The AAA+ (ATPases Associated with various cellular Activities) family member Rea1 (or Midasin) consists of nearly 5000 amino acids and generates force to mechanically remove assembly factors. Rea1 consists of an N-terminal α-helical domain (NTD), a ring of six AAA+ domains, and the C-terminal tail. The Rea1 tail is subdivided into an α-helical linker region, a D/E-rich region, and a MIDAS (Metal-Ion-Dependent Adhesion Site) domain which is responsible for the interaction with the Ytm1 and Rsa4 substrates. Rea1 pulls out the Ytm1 complex to promote the transfer of pre-60S particles from the nucleolus to the nucleoplasm.

In order to gain insight into the molecular basis for MIDAS domain docking, we decided to determine the cryoEM structure of the Rea1_ΔAAA2L-H2α AMPPNP state. The overall resolution of the reconstruction was 7.8 Å. The reconstruction revealed a density consistent with a MIDAS domain in-between the AAA3 and AAA4 modules, above AAA2S and AAA3S, respectively. As in the case of the Rea1_ΔAAA2L-H2α APO state, docking of this structure into the Rsa4 containing pre-60S structure would place the MIDAS domain in close contact with its Rsa4 substrate. Since the auto-inhibitory AAA2L-H2α insert has been deleted, the presence of AMPPNP is able to induce movements between the AAA+ modules of the AAA+ ring. The NTD, AAA1, AAA6 and the linker can be superimposed as a single rigid body, whereas the AAA2-AAA5 part has moved. The most drastic difference is apparent for the AAA4 module. Since the AAA2L-H2α insert is no longer pushing against AAA4L, the AAA4 module is free to move towards the central pore of the ring. We interpret these densities as two α-helices of the previously disordered AAA4L-H2α insert. The consequence of the combined movements of the AAA4 and AAA3 modules is that their small domains, AAA3S and AAA2S, adopt the right orientation with respect to each other to from the MIDAS domain binding site.

> XXXXXXXXXXXXXXXXXXXXXXXXXXXXXXXXXXXXXXXXXXXXXXXXXXXXXXXXXXXXXXXXXXXXXXXXXXXXXXXXXXXXXXXXXXXXXXXXXXXXXXXXXXXXXXXXXXXXXXXXXXXXXXXXXXXXXXXXXXXXXXXXXXXXXXXXXXXXXXXXXXXXXXXXXXXXXXXXXXXXXXXXXXXXXXPSVPECFTIEKKSSYFIIEPQDLSTKVASICGVIVPKVHTIHDKVFYPLTFVPTHKTVSSLRQLGRKIQNSTPIMLIGKAGSGKTFLINELSKYMGCHDSIVKIHLGEQTDAKLLIGTYTSGDKPGTFEWRAGVLATAVKEGRWVLIEDIDKAPTDVLSILLSLLEKRELTIPSRGETVKAANGFQLISTVRINEDHQKDSSNKIYNLNMIGMRIWNVIELEEPSEEDLTHILAQKFPILTNLIPKLIDSYKNVKSIYMNTKFISLNKGAHTRVVSVRDLIKLCERLDILFKNNGINKPDQLIQSSVYDSIFSEAADCFAGAIGEFKALEPIIQAIGESLDIASSRISLFLTQHVPTLENLDDSIKIGRAVLLKEKLNIQKKSMNSTLFAFTNHSLRLMEQISVCIQMTEPVLLVGETGTGKTTVVQQLAKMLAKKLTVINVSQQTETGDLLGGYKPVNSKTVAVPIQENFETLFNATFSLKKNEKFHKMLHRCFNKNQWKNVVKLWNEAYKMAQSILKITNTENENENAKKKKRRLNTHEKKLLLDKWADFNDSVKKFEAQSSSIENSFVFNFVEGSLVKTIRAGEWLLLDEVNLATADTLESISDLLTEPDSRSILLSEKGDAEPIKAHPDFRIFACMNPATDVGKRDLPMGIRSRFTEIYVHSPERDITDLLSIIDKYIGKYSVSDEWVGNDIAELYLEAKKLSDNNTIVDGSNQKPHFSIRTLTRTLLYVTDIIHIYGLRRSLYDGFCMSFLTLLDQKSEAILKPVIEKFTLGRLKNVKSIMSQTPPSPGPDYVQFKHYWMKKGPNTIQEQAHYIITPFVEKNMMNLVRATSGKRFPVLIQGPTSSGKTSMIKYLADITGHKFVRINNHEHTDLQEYLGTYVTDDTGKLSFKEGVLVEALRKGYWIVLDELNLAPTDVLEALNRLLDDNRELFIPETQEVVHPHPDFLLFATQNPPGIYGGRKILSRAFRNRFLELHFDDIPQDELEIILRERCQIAPSYAKKIVEVYRQLSIERSASRLFEQKNSFATLRDLFRWALRDAVGYEQLAASGYMLLAERCRTPQEKVTVKKTLEKVMKVKLDMDQYYASLEDKSLEAIGSVTWTKGMRRLSVLVSSCLKNKEPVLLVGETGCGKTTICQLLAQFMGRELITLNAHQNTETGDILGAQRPVRNRSEIQYKLIKSLKTALNIANDQDVDLKELLQLYSKSDNKNIAEDVQLEIQKLRDSLNVLFEWSDGPLIQAMRTGNFFLLDEISLADDSVLERLNSVLEPERSLLLAEQGSSDSLVTASENFQFFATMNPGGDYGKKELSPALRNRFTEIWVPSMEDFNDVNMIVSSRLLEDLKDLANPIVKFSEWFGKKLGGGNATSGVISLRDILAWVEFINKVFPKIQNKSTALIQGASMVFIDALGTNNTAYLAENENDLKSLRTECIIQLLKLCGDDLELQQIETNEIIVTQDELQVGMFKIPRFPDAQSSSFNLTAPTTASNLVRVVRAMQVHKPILLEGSPGVGKTSLITALANITGNKLTRINLSEQTDLVDLFGADAPGERSGEFLWHDAPFLRAMKKGEWVLLDEMNLASQSVLEGLNACLDHRGEAYIPELDISFSCHPNFLVFAAQNPQYQGGGRKGLPKSFVNRFSVVFIDMLTSDDLLLIAKHLYPSIEPDIIAKMIKLMSTLEDQVCKRKLWGNSGSPWEFNLRDTLRWLKLLNQYSICEDVDVFDFVDIIVKQRFRTISDKNKAQLLIEDIFGKFSTKENFFKLTEDYVQINNEVALRNPHYRYPITQNLFPLECNVAVYESVLKAINNNWPLVLVGPSNSGKTETIRFLASILGPRVDVFSMNSDIDSMDILGGYEQVDLTRQISYITEELTNIVREIISMNMKLSPNATAIMEGLNLLKYLLNNIVTPEKFQDFRNRFNRFFSHLEGHPLLKTMSMNIEKMTEIITKEASVKFEWFDGMLVKAVEKGHWLILDNANLCSPSVLDRLNSLLEIDGSLLINECSQEDGQPRVLKPHPNFRLFLTMDPKYGELSRAMRNRGVEIYIDELHSRSTAFDRLTLGFELGENIDFVSIDDGIKKIKLNEPDMSIPLKHYVPSYLSRPCIFAQVHDILLLSDEEPIEESLAAVIPISHLGEVGKWANNVLNCTEYSEKKIAERLYVFITFLTDMGVLEKINNLYKPANLKFQKALGLHDKQLTEETVSLTLNEYVLPTVSKYSDKIKSPESLYLLSSLRLLLNSLNALKLINEKSTHGKIDELTYIELSAAAFNGRHLKNIPRIPIFCILYNILTVMSENLKTESLFCGSNQYQYYWDLLVIVIAALETAVTKDEARLRVYKELIDSWIASVKSKSDIEITPFLNINLEFTDVLQLSRGHSITLLWDIFRKNYPTTSNSWLAFEKLINLSEKFDKVRLLQFSESYNSIKDLMDVFRLLNDDVLNNKLSEFNLLLSKLEDGINELELISNKFLNKRKHYFADEFDNLIRYTFSVDTAELIKELAPASSLATQKLTKLITNKYNYPPIFDVLWTEKNAKLTSFTSTIFSSQFLEDVVRKSNNLKSFSGNQIKQSISDAELLLSSTIKCSPNLLKSQMEYYKNMLLSWLRKVIDIHVGGDCLKLTLKELCSLIEEKTASETRVTFAEYIFPALDLAESSKSLEELGEAWITFGTGLLLLFVPDSPYDPAIHDYVLYDLFLKTKTFSQNLMKSWRNVRKVISGDEEIFTEKLINTISDDDAPQSPRVYRTGMSIDSLFDEWMAFLSSTMSSRQIKELVSSYKCNSDQSDRRLEMLQQNSAHFLNRLESGYSKFADLNDILAGYIYSINFGFDLLKLQKSKDRASFQISPLWSMDPINISCAENVLSAYHELSRFFKKGDMEDTSIEKVLMYFLTLFKFHKRDTNLLEIFEAALYTLYSRWSVRRFRQEQEENEKSNMFKFNDNSDDYEADFRKLFPDYEDTALVTNEKDISSPENLDDIYFKLADTYISVFDKDHDANFSSELKSGAIITTILSEDLKNTRIEELKSGSLSAVINTLDAETQSFKNTEVFGNIDFYHDFSIPEFQKAGDIIETVLKSVLKLLKQWPEHATLKELYRVSQEFLNYPIKTPLARQLQKIEQIYTYLAEWEKYASSEVSLNNTVKLITDLIVSWRKLELRTWKGLFNSEDAKTRKSIGKWWFYLYESIVISNFVSEKKETAPNATLLVSSLNLFFSKSTLGEFNARLDLVKAFYKHIQLIGLRSSKIAGLLHNTIKFYYQFKPLIDERITNGKKSLEKEIDDIILLASWKDVNVDALKQSSRKSHNNLYKIVRKYRDLLNGDAKTIIEAGLLYXXXXXXXXXXXXXXXXXXXXXXXXXXXXXXXRNIDTVASNMDSYLEKISSQEFPNFADLASDFYAEAERLRKETPNVYTKENKKRLAYLKTQKSKLLGDALKELRRIGLKVNFREDIQKVQSSTTTILANIAPFNNEYLNSSDAFFFKILDLLPKLRSAASNPSDDIPVAAIERGMALAQSLMFSLITVRHPLSEFTNDYCKINGMMLDLEHFTCLKGDIVHSSLKANVDNVRLFEKWLPSLLDYAAQTLSVISKYSATSEQQKILLDAKSTLSSFFVHFNSSRIFDSSFIESYSRFELFINELLKKLENAKETGNAFVFDIIIEWIKANKGGPIKKEQKRGPSVEDVEQAFRRTFTSIILSFQKVIGDGIESISETDDNWLSASFKKVMVNVKLLRSSVVSKNIETALSLLKDFDFTTTESIYVKSVISFTLPVITRYYNAMTVVLERSRIYYTNTSRGMYILSTILHSLAKNGFCSPQPPSEEVDDKNLQEGTGLGDGEGAQNNNKDVEQDEDLTEDAQNENKEQQDKDERDDENEDDAVEMEGDMAGELEDLSNGEENDDEDTDSEEEELDEEIDDLNEDDPNAIDDKMWDDKASDNSKEKDTDQNLDGKNQEEDVQAAENDEQQRDNKEGGDEDPNAPEDGDEEIENDENAEEENDVGEQEDEVKDEEGEDLEANVPEIETLDLPEDMNLDSEHEESDEDVDMSDGMPDDLNKEEVGNEDEEVKQESGIESDNENDEPGPEEDAGETETALDEEEGAEEDVDMTNDEGKEDEENGPEEQAMSDEEELKQDAAMEENKEKGGEQNTEGLDGVEEKADTEDIDQEAAVQQDSGSKGAGADATDTQEQDDVGGSGTTQNTYEEDQEDVTKNNEESREEATAALKQLGDSMKEYHRRRQDIKEAQTNGEEDENLEKNNERPDEFEHVEGANTETDTQALGSATQDQLQTIDEDMAIDDDREEQEVDQKELVEDADDEKMDIDEEEMLSDIDAHDANNDVDSKKSGFIGKRKSEEDFENELSNEHFSADQEDDSEIQSLIENIEDNPPDASASLTPERSLEESRELWHKSEISTADLVSRLGEQLRLILEPTLATKLKGDYKTGKRLNMKRIIPYIASQFRKDKIWLRRTKPSKRQYQIMIALDDSKSMSESKCVKLAFDSLCLVSKTLTQLEAGGLSIVKFGENIKEVHSFDQQFSNESGARAFQWFGFQETKTDVKKLVAESTKIFERARAMVHNDQWQLEIVISDGICEDHETIQKLVRRARENKIMLVFVIIDGITSNESILDMSQVNYIPDQYGNPQLKITKYLDTFPFEFYVVVHDISELPEMLSLILRQYFTDLASS> IVCHTTA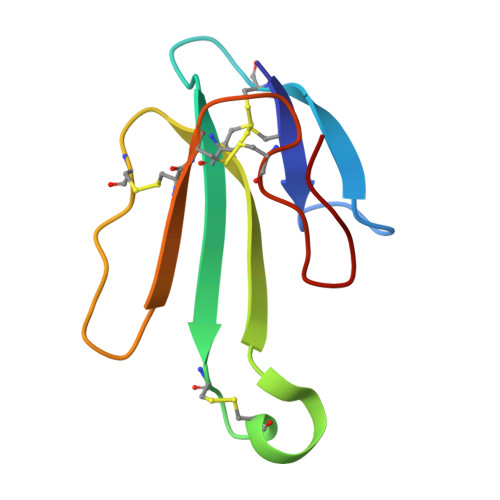TSPISAVTCPPGENLCYRKMWCDAFCSSRGKVVELGCAATCPSKKPYEEVTCCSTDKCNPHPKQRPG>MAKSGNYSYKRWVFTINNPTFEDYVHVLEFCTLDNCKFAIVGEEKGANGTPHLQGFLNLRSNA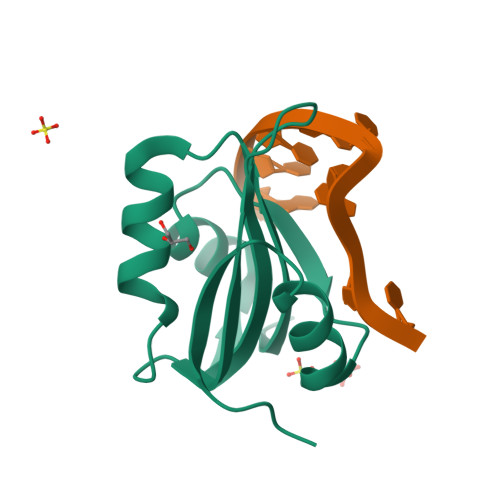RAAALEESLGGRAWLSRARGSDEDNEEFCAKESTYLRVGEPVSKGRSS[2x]> MPFVNKQFNYKDPVNGVDIAYIKIPNAGQMQPVKAFKIHNKIWVIPERDTFTNPEEGDLNPPPEAKQVPVS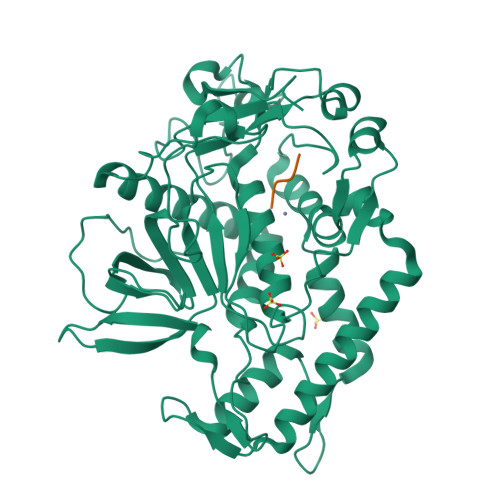YYDSTYLSTDNEKDNYLKGVTKLFERIYSTDLGRMLLTSIVRGIPFWGGSTIDTELKVIDTNCINVIQPDGSYRSEELNLVIIGPSADIIQFECKSFGHEVLNLTRNGYGSTQYIRFSPDFTFGFEESLEVDTNPLLGAGKFATDPAVTLAHELIHAGHRLYGIAINPNRVFKVNTNAYYEMSGLEVSFEELRTFGGHDAKFIDSLQENEFRLYYYNKFKDIASTLNKAKSIVGTTASLQYMKNVFKEKYLLSEDTSGKFSVDKLKFDKLYKMLTEIYTEDNFVKFFKVLNRKTYLNFDKAVFKINIVPKVNYTIYDGFNLRNTNLAANFNGQNTEINNMNFTKLKNFTGLFEHHHHHH;> RRGFX> TNRTPKQKIEQQIDSLLKDKKATVGVAVLANDETVAVYNNQIHFPLLSVFKFHVGLAVLDKMDKGHIALDSLIEVKSSQLKSNTYSPLRDKFPDQDITISLGELLKYTISKSDNNTCDILIEYVGGIDQVNEYVKSLGIKDCNLAATETLMHTSGDTDLNWSTPEEVVRLLNIADKQPLFGTQYKDFLQAIMQET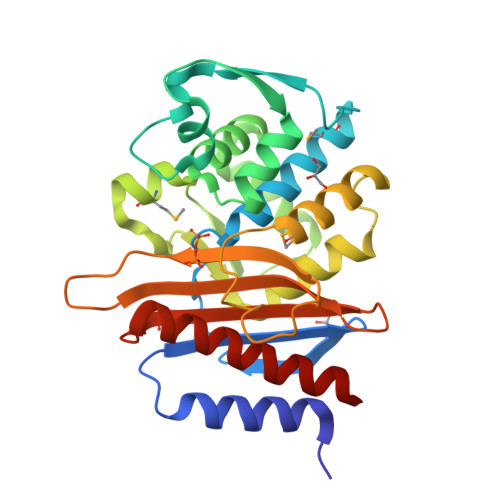STGKDKLKGQLPADVIVGHKTGSSDRTPEGIKIADNDAGFVILPNGQKYYIAVFVMESQETDADNAAIIASISKIVYDTLNSDIQ>[2x]QAGVQKVRAWGPGLETGQVGKSADFVVEAIGTEVGTLGFSIEGPSQAKIECDDKGDGSCDVRYWPTEPGEYAVHVICDDEDIRDSPFIAHILPAPPDCF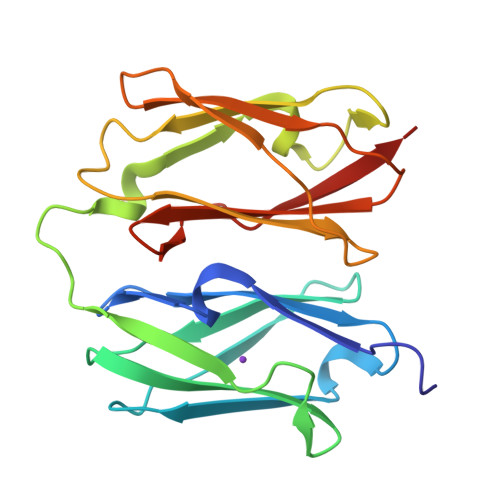PDKVKAFGPGLEPTGCIVDKPAEFTIDARAAGKGDLKLYAQDADGCPIDIKVIPNGDGTFRCSYVPTKPIKHTIIISWGGVNVPKSPFRVNVGEG> GPDEIDLSALRDPAGIFELVELVGNGTYGQVYKGRHVKTG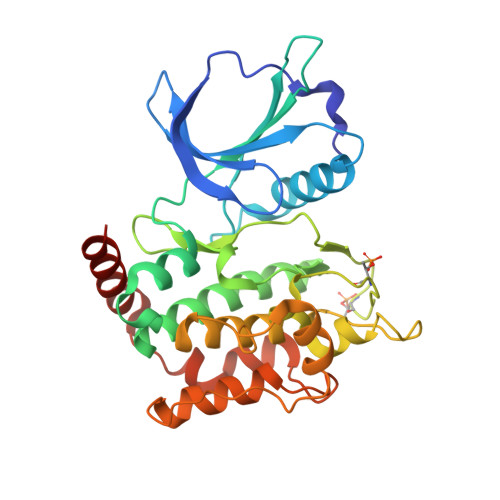QLAAIKVMDVTGDEEEEIKQEINMLKKYSHHRNIATYYGAFIKKNPPGMDDQLWLVMEFCGAGSVTDLIKNTKGNTLKEEWIAYICREILRGLSHLHQHKVIHRDIKGQNVLLTENAEVKLVDFGVSAQLDRTVGRRNTFIGTPYWMAPEVIACDENPDATYDFKSDLWSLGITAIEMAEGAPPLCDMHPMRALFLIPRNPAPRLKSKKWSKKFQSFIESCLVKNHSQRPATEQLMKHPFIRDQPNERQVRIQLKDHIDRTKKKRG> SKYGLQDSDE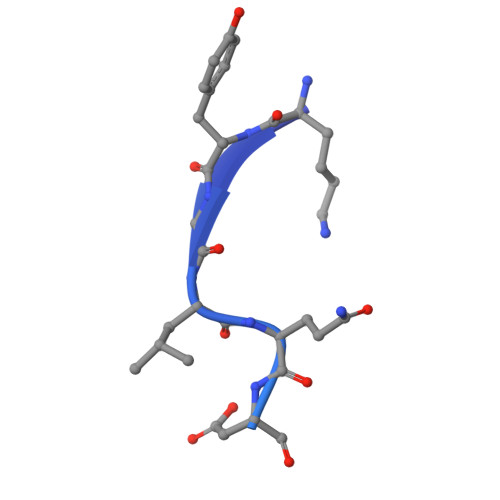EEEEHPSKTSTKKLKTAPLPPASQTTPLQMALNGKPAPPPQVEKKGQLEHHHHH> MSTMSTPAAEQRKLVEQLMGRDFSFRHNRYSHQKRDLGLHDP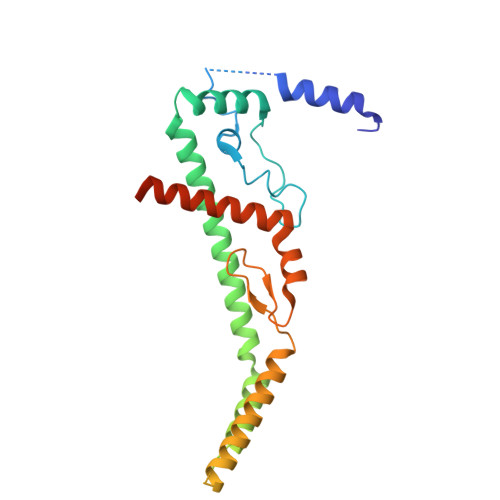KICKSYLVGECPYDLFQGTKQSLGKCPQMHLTKHKIQYEREVKQGKTFPEFEREYLAILSRFVNECNGQISVALQNLKHTAEERMKIQQVTEELDVLDVRIGLMGQEIDSLIRADEVSMGMLQSVKLQELISKRKEVAKRVRNITENVGQSAQQKLQVCEVCGAYLSRLDTDRRLADHFLGKIHLGYVKMREDYDRLMKNNRTTNASKTATTLPGRRFV> MFADVETTCCARRTLTTIDEVPGMADETALLDWLGTMREKQPVWQDRYGVWHVFRHADVQTVLRDTATFSSDPTRVIEGASPTPGMIHEIDPPE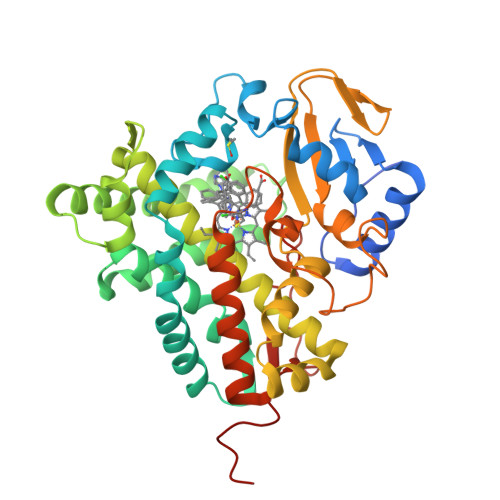HRALRKVVSSAFTPRTISDLEPRIRDVTRSLLADAGESFDLVDVLAFPLPVTIVAELLGLPPMDHEQFGDWSGALVDIQMDDPTDPALAERIADVLNPLTAYLKARCAERRADPGDDLISRLVLAEVDGRALDDEEAANFSTALLLAGHITTTVLLGNIVRTLDEHPAHWDAAAEDPGRIPAIVEEVLRYRPPFPQMQRTTTKATEVAGVPIPADVMVNTWVLSANRDSDAHDDPDRFDPSRKSGGAAQLSFGHGVHFCLGAPLARLENRVALEEIIARFGRLTVDRDDERLRHFEQIVLGTRHLPVLAGSSPRQSA>MLSRKGIIPEEYVLTRLAEDPAKPRYRARQRRARFVSKKGNCNVAHKNIREQGRFLQDVFTTLVDLKWPHTLLIFTMSFLCSWLLFAMAWWLIAFAHGDLAPSEGTAEPCVTSIHSFSSAFLFSIEVQVTIGFGGRMVTEECPLAILILIVQNIVGLMINAIMLGSIFMKTAQAHRRAETLIFSKHAVIALRHGRLCFMLRVGDLRKSMIISATIHMQVVRKTTSPEGEVVPLHQVDIPMENGVGGNSIFLVAPLIIYHVIDANSPLYDLAPSDLHHHQDLEIIVILEGVVETTGITTQARTSYLADEILWGQRFVPIVAEEDGRYSVDYSKFDNTVKVPTPLCTARQLDEDHSLLEALTLASARGPLRKRSVPMAKAKPKFSISPDSLS[4x];> MGPLAFCGSENHSAAYRVDQGVLNNGCFVDALNVVPHVFLLFITFPILFIGWGSQSSKVHIHHSTWLHFPGHNLRWILTFMLLFVLVCEIAEGILSDGVTESHHLHLYMPAGMAFMAAVTSVVYYHNIETSNFPKLLIALLVYWTLAFITKTIKFVKFLDHAIGFSQLRFCLTGLLVILYGMLLLVEVNVIRVRRYIFFKTPREVKPPEDLQDLGVRFLQPFVNLLSKGTYWWMNAFIKTAHKKPIDLRAIGKLPIAMRALTNYQRLCEAFDAQVRKDIQGTQGARAIWQALSHAFGRRLVLSSTFRILADLLGFAGPLCIFGIVDHLGKENDVFQPKTQFLGVYFVSSQEFLANAYVLAVLLFLALLLQRTFLQASYYVAIETGINLRGAIQTKIYNKIMHLSTSNLSMGEMTAGQICNLVAIDTNQLMWFFFLCPNLWAMPVQIIVGVILLYYILGVSALIGAAVIILLAPVQYFVATKLSQAQRSTLEYSNERLKQTNEMLRGIKLLKLYAWENIFRTRVETTRRKEMTSLRAFAIYTSISIFMNTAIPIAAVLITFVGHVSFFKEADFSPSVAFASLSLFHILVTPLFLLSSVVRSTVKALVSVQKLSEFLSSAEIREEQCAPHEPTPQGPASKYQAVPLRVVNRKRPAREDCRGLTGPLQSLVPSADGDADNCCVQIMGGYFTWTPDGIPTLSNITIRIPRGQLTMIVGQVGCGKSSLLLAALGEMQKVSGAVFWSSLPDSEIGEDPSPERETATDLDIRKRGPVAYASQKPWLLNATVEENIIFESPFNKQRYKMVIEACSLQPDIDILPHGDQTQIGERGINLSGGQRQRISVARALYQHANVVFLDDPFSALDIHLSDHLMQAGILELLRDDKRTVVLVTHKLQYLPHADWIIAMKDGTIQREGTLKDFQRSECQLFEHWKTLMNRQDQELEKETVTERKATEPPQGLSRAMSSRDGLLQDEEEEEEEAAESEEDDNLSSMLHQRAEIPWRACAKYLSSAGILLLSLLVFSQLLKHMVLVAIDYWLAKWTDSALTLTPAARNCSLSQECTLDQTVYAMVFTVLCSLGIVLCLVTSVTVEWTGLKVAKRLHRSLLNRIILAPMRFFETTPL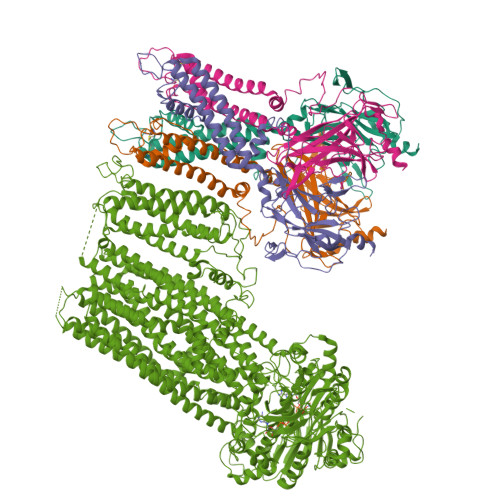GSILNRFSSDCNTIDQHIPSTLECLSRSTLLCVSALAVISYVTPVFLVALLPLAIVCYFIQKYFRVASRDLQQLDDTTQLPLLSHFAETVEGLTTIRAFRYEARFQQKLLEYTDSNNIASLFLTAANRWLEVRMEYIGACVVLIAAVTSISNSLHRELSAGLVGLGLTYALMVSNYLNWMVRNLADMELQLGAVKRIHGLLKTEAESYEGLLAPSLIPKNWPDQGKIQIQNLSVRYDSSLKPVLKHVNALIAPGQKIGICGRTGSGKSSFSLAFFRMVDTFEGHIIIDGIDIAKLPLHTLRSRLSIILQDPVLFSGTIRFNLDPERKCSDSTLWEALEIAQLKLVVKALPGGLDAIITEGGENFSQGQRQLFCLARAFVRKTSIFIMDEATASIDMATENILQKVVMTAFADRTVVTIAHRVHTILSADLVIVLKRGAILEFDKPEKLLSRKDSVFASFVRADK> AE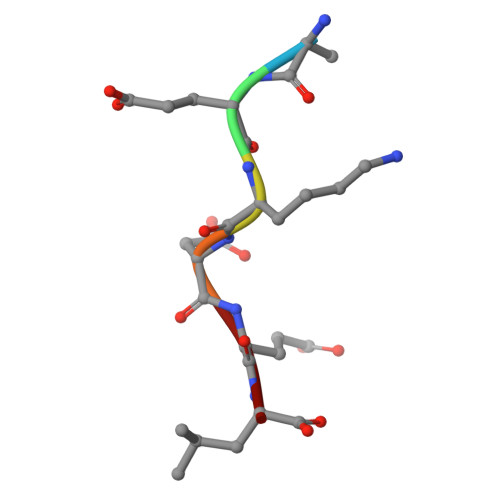KDEL> MKKQKSKKTVSKTSGLKEALSVQGTVIMTSFGKGNMANLSYKIPSSQKPQNLNSSAGLKNVEVSGKKIKFQGRHPKIATTDNPLFKPQPGMDLLCLKDKLEMHYFGKTFDDNIHIQLIYQILDIEKILAVHVNNIVFTLDNVLHPQKEELTEDFIGAGGWRINLDYQTLRGQTNKYDRFKNYIKRKELLYFGEAFYHENERRYEEDIFAILTLLSALAQFCFASDLSSDESDHVNSFWLYQLEDQLSDEFKETLSILWEEVTERIDSEFLKTNTVNLHILCHVFPKESKETIVRAYYEFLIKKSFKNMGFSIKKLRE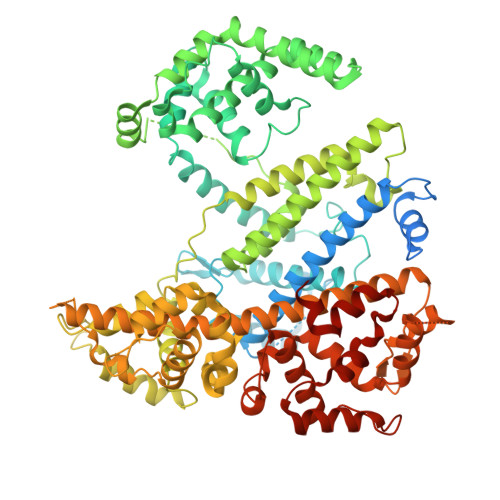IMLEQSDLKSFKEDKYNSVRAKLYKLFDFIITYYYDHHAFEKEALVSSLRSSLTEENKEEIYIKTARTLASALGADFKKAAADVNAKNIRDYQKKANDYRISFEDIKIGNTGIGYFSELIYMLTLLLDGKEINDLLTTLINKFDNIISFIDILKKLNLEFKFKPEYADFFNMTNCRYTLEELRVINSIARMQKPSADARKIMYRDALRILGMDNRPDEEIDRELERTMPVGADGKFIKGKQGFRNFIASNVIESSRFHYLVRYNNPHKTRTLVKNPNVVKFVLEGIPETQIKRYFDVCKGQEIPPTSDKSAQIDVLARIISSVDYKIFEDVPQSAKINKDDPSRNFSDALKKQRYQAIVSLYLTVMYLITKNLVYVNSRYVIAFHCLERDAFLHGVTLPKMNKKIVYSQLTTHLLTDKNYTTYGHLKNQKGHRKWYVLVKNNLQNSDITAVSSFANIVAAISVVRNSNEYISGIGELHSYFELYHYLVQSMIAKNNWYDTSHQPKTAEYLNNLKKHHTYCKDFVKAYCIPFGYVVPRYKNLTINELFDRNNPNPEPKEEV> GPLGSAYMSRRESINPWILTGFADAEGSFLLRIRNNNKSSVGYSTELGFQITLHNKDKSILENIQSTWKVGVIANSGDNAVSLKVTRFEDLKVIIDHFEKYPLITQKLGDYMLFKQAFCVMENKEHLKINGIKELVRIKAKLNWGLTDELKKAFPEIISKERSLINKNIPNFKWLAGFTSGEGCFFVNLIKSKSKL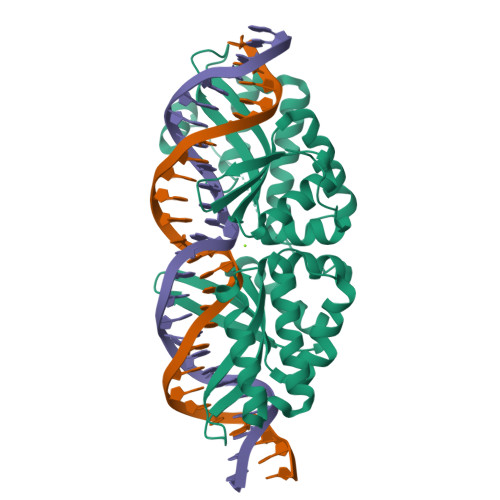GVQVQLVFSITQHIKDKNLMNSLITYLGCGYIKEKNKSEFSWLDFVVTKFSDINDKIIPVFQENTLIGVKLEDFEDWCKVAKLIEEKKHLTESGLDEIKKIKLNMNKGRVF> DNSNNPVGGNPIDNYGTEHAPLLKEDNQYLVYQGERIVSFKDLLRRYQYLNSYWPQETGSGFRYYTLDSPGMPIYRGWDPNGIDQGQDSTAGNSPYNFCSMTL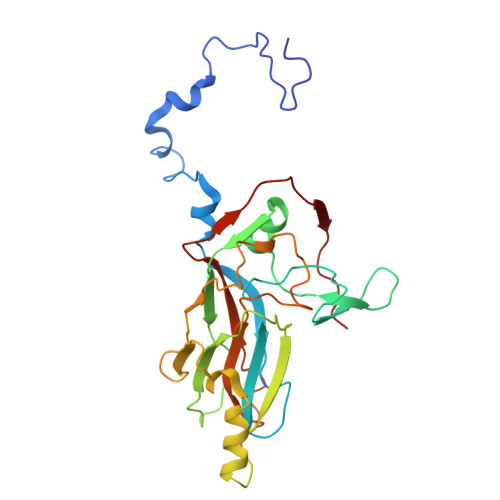LNYLAPAFVCQRGSLRHKWVTAGARVNSTASVLSATRHGVLFPLPLAETAHPLDNALVGDRRSELQEMQRSRLNGTAITPVRLNNTLEIELPYYSIGQRFHASRFLDLAGTGDTQGVEIACEISDGGNDANYRLDQFVSVGEDFTLGMFVGAPIMYFYNDPTAT>MSLTNVKPLIKESHHIILADDGDICIGEIPGVSQVINDPPSWVRPALAKMDGKRTVPRIFKELVSEGVQIESEHLEGLVAGLAERKLLQDNSFFSKVLSGEEVERYNRQILQFSLIDADNQHPFVYQERLKQSKVAIFGMGGWGTWCALQLAMSGIGTLRLIDGDDVELSNINRQVLYRTDDVGKNKVDAAKDTILAYNENVHVETFFEFASPDRARLEELVGDSTFIILAWAALGYYRKDTAEEIIHSIAKDKAIPVIELGGDPLEISVGPIYLNDGVHSGFDEVKNSVKDKYYDSNSDIRKFQEARLKHSFIDGDRKVNAWQSAPSLSIMAGIVTDQVVKTITGYDKPHLVGKKFILSLQDFRSREEEIFKLEHHHHH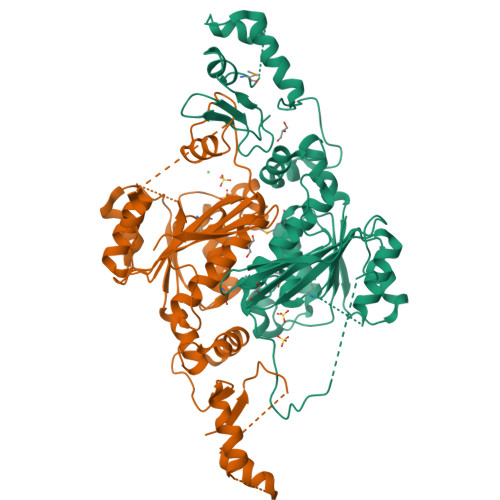H[2x]AChBPs are homopentameric, water-soluble homologs of the ligand-binding domain of LGICs and well-established structural surrogates for nicotinic acetylcholine receptors (nAChR). Importantly, AChBPs can bind nAChR-specific ligands and induce similar conformational changes as in the membrane bound receptors. LGICs are activated by ligands binding at subunit interfaces of their extracellular domains, thereby inducing conformational changes that affect the structure of a central pore and its ability to transport ions through the membrane. Additional density was found in all structures at the interface between the subunits in the orthosteric agonist and antagonist binding site, next to loop C in which the respective ligands could be modelled.

The sensorgrams had concentration dependent distortions in both the association and dissociation phases, with a negative slope at steady state and signals below baseline once the ligand injection was stopped. Surface Acoustic Wave (SAW) biosensor technology was used to confirm that distortions observed in SPR biosensor data for interactions between compounds VUF6105, VUF22430, and VUF24234, and AChBP indeed result from ligand-induced conformational changes. The three VUF compounds resulted in significant ΔSHG responses with all labelling variants, with VUF22430 giving very high signals. Similarly, VUF6105 resulted in a significant compaction, while VUF24234 resulted in an expansion. As seen from the different conformational changes induced by each compound, this analysis revealed that the binding modes of VUF6105 and VUF24234 are different. The unit cell was comprised of two or four pentamers of Ls-AChBP in the presence of FL1613, FL1856, FL1888, FL3044, VUF24234 and VUF6105. Notably, binding of FL1888, VUF24234 and VUF6105 results in a movement of the loop closer to the compound, while binding of FL1856, FL3044, FL1613 and FL1909 does not have the same effect. The violin plot revealed that conformational changes in loop C occurred to a higher degree in the AChBP structures with compounds FL1888, VUF24234 and VUF6105 than in the other structures. This correlated with the results from the SPR, SAW and SHG biosensor experiments, which all indicated conformational changes in AChBP upon binding of these compounds.

>FDRADILYNIRQTSRPDVIPTQRDRPVAVSVSLKFINILEVNEITNEVDVVFWQQTTWSDRTLAWNSSHSPDQVSVPISSLWVPDLAAYNAISKPEVLTPQLARVVSDGEVLYMPSIRQRFSCDVSGVDTESGATCRIKIGSWTHHSREISVDPTTENSDDSEYFSQYSRFEILDVTQKKNSVTYSCCPEAYEDVEVSLNFRKKGR[10x]> SGIRELNLTKEQHEWLNGWLELWGAWVYSGRLEKRMSSVIAKFMESVEPGRVMTRPMCNDDDGMLISQVVDSVMYIDKKAFGILLS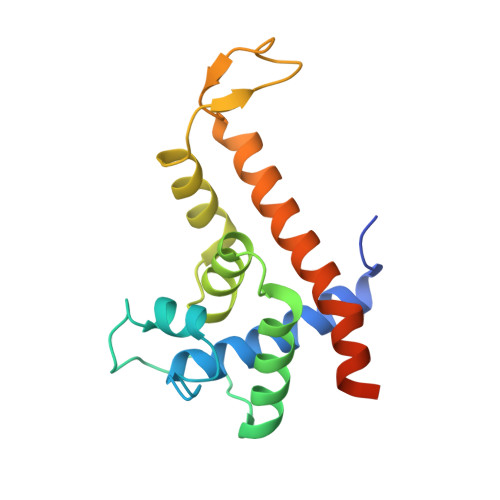YYAHGSSKHAIASYYHRVARPRKMLCRGGGRIQKPSLATCRREVDEILNASLFMIYPVLDSAFKNRKRVEKIKHVA>[4x]GMAYEQFAYVYDELMQDVPYPE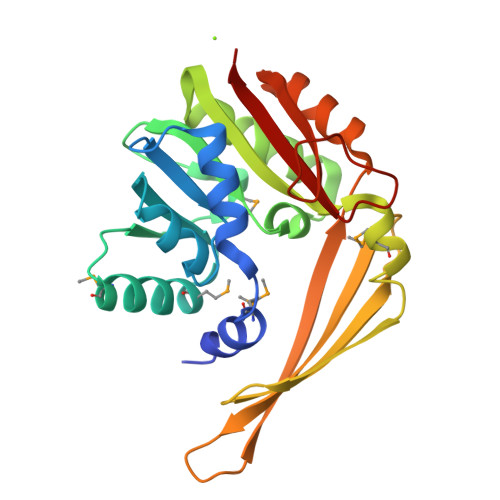WVAWVLEQVEPGKRIADIGCGTGTATLLLADHYEVTGVDLSEEMLEIAQEKAMETNRHVDFWVQDMRELELPEPVDAITILCDSLNYLQTEADVKQTFDSAARLLTDGGKLLFDVHSPYKMETLFNGKTYATHAEQSSYIWFADPGEEPLSVVHELTFFIEGEDGRYDRVDETHHQRTYPPEQYITWLREAGFRVCAVTGDFKSDAPTETAERIFFVAEKI> ALWQFNGMIKCKIPSSEPLLDFNNYGCYCGLGGSGTPVDDLDRCCQTNDNCYKQ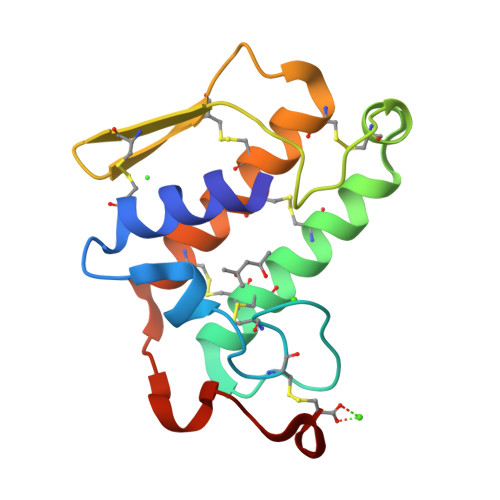AKKLDSCKVLVDNPYTNNYSYSCSNNEITCSSENNACEAFICNCDRNAAICFSKVPYNKEHKNLDKKNC>[2x]MSNLLTVHQNLPALPVDATSDEVRKNLMDMFRDRQAFSEHTWKMLLSVCRSWAAWCKLNNRKWFPAEPEDVRDYLLYLQARGLAVKTIQQHLGQLNMLHRRSGLPRPSDSNAVSLVMRRIRKENVDAGERAKQALAFERTDFDQVRSLMENSDRCQDIRNLAFLGIAYNTLLRIAEIARIRVKDISRTDGGRMLIH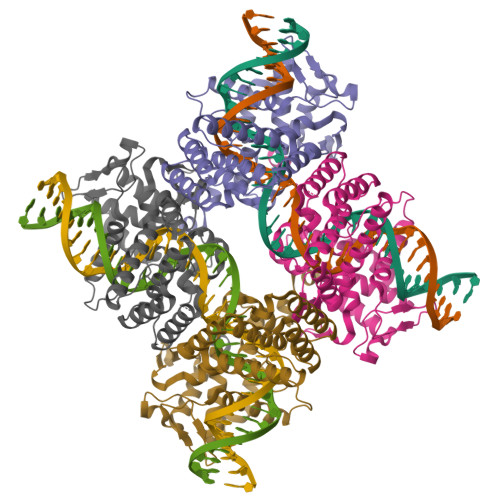IGRTATLVSTAGVEKALSLGVTKLVERWISVSGVADDPNNYLFCRVRKNGVAAPSATSQLSTRALEGIFEATHRLIYGAKDDSGQRYLAWSGHSARVGAARDMARAGVSIPEIMQAGGWTNVNIVMNYIRNLDSETGAMVRLLEDGD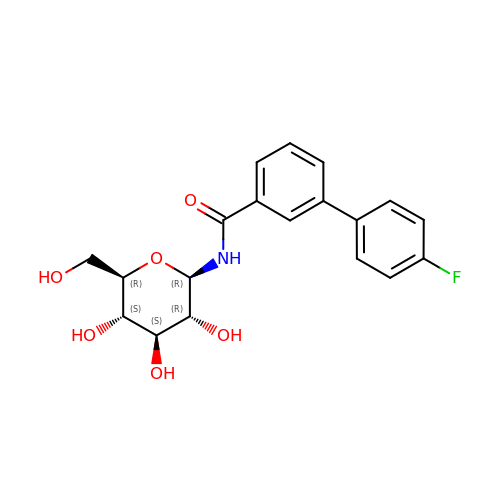3-(4-fluorophenyl)-~{N}-[(2~{R},3~{R},4~{S},5~{S},6~{R})-6-(hydroxymethyl)-3,4,5-tris(oxidanyl)oxan-2-yl]benzamide | C19 H20 F N O6 | ZNFXGMNTWYBCJQ-OGJJZOIMSA-N E. coli cells containing CL-GESSNitR-L117F were transformed with the pET28a(+) plasmid encoding an individual ORF to detect the fluorescence signal corresponding to the conversion of 6-ACA to ε-caprolactam. We found that an ORF encoding 3-hydroxybutyrate dehydrogenase from Citrobacter freundii (CF3HBD) was positive for this activity (number 2 in Fig. 4b). Basically, the screened CF3HBDs belong to the NAD(P)H-dependent short-chain dehydrogenase family, and they have cyclization activity as unexpected promiscuous activity. d-3-Hydroxybutyrate dehydrogenase catalyzed the reversible and stereospecific oxidation of d-3-hydroxybutyric acid to acetoacetate using NAD+ as a coenzyme. The resulting isolate, CF3HBD is a unique biocatalyst with lactam-synthesizing activity as promiscuous activity that does not require a cofactor or energy source in an in vitro system. In addition, we found that CF3HBD could catalyze the degradation of the cyclic amide group in ε-caprolactam, generating 6-ACA as a reaction product.

To further characterize the cyclization activity, we determined the crystal structure of CF3HBD in complex with NAD+ at a resolution of 2.29 Å. We found that the asymmetric unit had a tetramer structure with two NAD+-free subunits. Nearly all of the residues were well defined in the electron-density map, except the unidentified electron density located in the pocket near the nicotinamide group of NAD+, which corresponded to the active site of CF3HBD. Based on its position, this density could represent a molecule of ε-caprolactam transiently captured by the enzyme during crystal packing. Molecular docking of CF3HBD with 6-ACA and ε-caprolactam in the unidentified electron density was achieved using the holo form of CF3HBD. The docking results suggested that 10 residues (Q91, S139, V140, H141, K149, Y152, Q193, W184, V190, and Q193) located within 4.0 Å of the center of the docked substrate are active-site residues. Alanine substitution of the catalytic residues, such as Q91, S139, and H141 completely abolished catalytic activity towards both 3-hydroxybutyric acid and 6-ACA, which suggested that dehydrogenation activity and cyclization activity share catalytic site. Alanine substitution at V140, Y152, and W184 resulted in lack of activity towards 3-hydroxybutyric acid, whereas these mutants showed cyclization activities for 6-ACA of more than 80%. Interestingly, the Y152A mutant showed the highest cyclization activity, with a three-fold increase, for 6-ACA. The Y152A mutant had about 3.4-fold higher catalytic efficiency than that of wild-type enzyme. This result suggested that an alanine residue may be preferred rather than the bulky aromatic amino acid to allow 6-ACA in the active site, but not 3-hydroxybutyric acid.

>MNLTGKTALVTGSTSGIGLGIAQVLAQAGATLILNGFGDVDAAKDAVAQYGKTPGYHGADLSDEAQIADMMRYAESEFGGVDILINNAGIQHVSPIETFPVDKWNAIIAINLSSVFHTTRLALPGMRARNWGRIINIASVHGLVASKEKSAYVAAKHGVVGLTKTIALETAQTEITCNALCPGWVLTPLVQQQIDKRIAEGAEPEAARDALLAEKQPSREFVTPEQLGNLALFLCSDGAAQVRGVAWNMDGGWVAQ[4x]>[2x]MNPAAEAEFNILLATDSYKVTHYKQYPPNTSKVYSY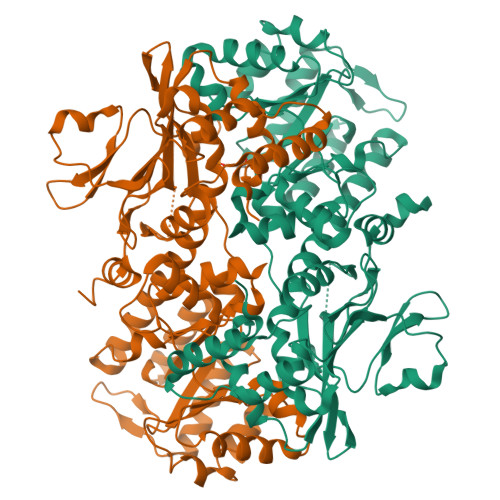FECREKKTENSKLRKVKYEETVFYGLQYILNKYLKGKVVTKEKIQEAKDVYKEHFQDDVFNEKGWNYILEKYDGHLPIEIKAVPEGFVIPRGNVLFTVENTDPECYWLTNWIETILVQSWYPITVATNSREQKKILAKYLLETSGNLDGLEYKLRDFGYRGVSSQETAGIGASAHLVNFKGTDTVAGLALIKKYYGTKDPVPGYSVPAAEHSTITAWGKDHEKDAFEHIVTQFSSVPVSVVSDSYDIYNACEKIWGEDLRHLIVSRSTQAPLIIRPDSGNPLDTVLKVLEILGKKFPVTENSKGYKLLPPYLRVIQGDGVDINTLQEIVEGMKQKMWSIENIAFGSGGGLLQKLTRDLLNCSFKCSYVVTNGLGINVFKDPVADPNKRSKKGRLSLHRTPAGNFVTLEEGKGDLEEYGQDLLHTVFKNGKVTKSYSFDEIRKNAQLNIELEAAHHLEHHHHHHHH> MDEEPPFNLALNVYKGPASIPHASAEVFGAFFLATNTALLAHMFPGKLFGSELHVRKWDPDYLASCCNEQGMRREALSGKKPNLWLLGGGPRLVNDSWERMW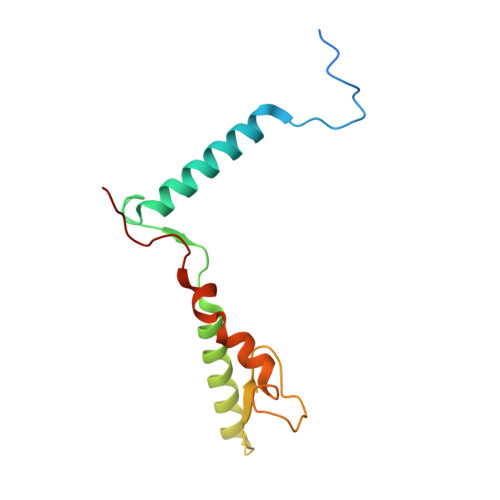WNNLHWKRWKVPRTGPAFPQDMYWQ>GIIEFHVIGNSLTPKANRRVLLWLVGLQNVFSHQLPRMPKEYIARLVFDPKHKTLALIKDGRVIGGICFRMFPTQGFTEIVFCAVTSNEQVKGYGTH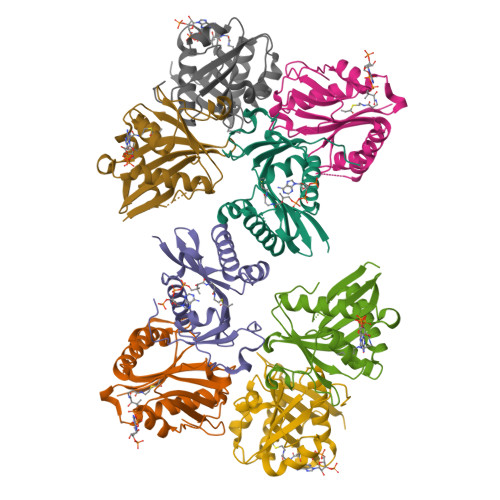LMNHLKEYHIKHNILYFLTYADEYAIGYFKKQGFSKDIKVPKSRYLGYIKDYEGATLMECELNPRIPYT[8x]>[3x]KPIEIIGAPFS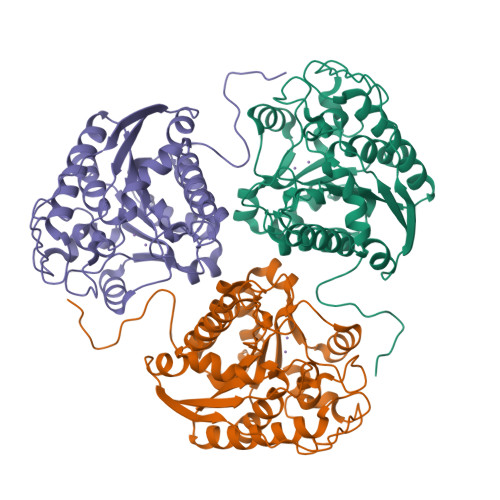KGQPRGGVEKGPAALRKAGLVEKLKETEYNVRDHGDLAFVDVPNDSPFQIVKNPRSVGKANEQLAAVVAETQKNGTISVVLGGDHSMAIGSISGHARVHPDLCVIWVDAHTDINTPLTTSSGNLDGQPVAFLLKELKGKFPDVPGFSWVTPCISAKDIVYIGLRDVDPGEHYIIKTLGIKYFSMTEVDKLGIGKVMEETFSYLLGRKKRPIHLSFDVDGLDPVFTPATGTPVVGGLSYREGLYITEEIYKTGLLSGLDIMEVNPTLGKTPEEVTRTVNTAVALTLSCFGTKREGNHKPETDYL> GSEFVKEHDWKKCDQSGFCRRNRAYADHALSAISWESPYKIAPETGSFKDGQYQAIILKTINDHGETVRLPLTVSFLESGTARVTIDEEKRQKGEIELRHDSKARKERYNEAEQWVIVGGMTLDKGAKVDYEDKTQMTVKYGPSSKFEATIKFAPFSIDFKRDGASHIKFNDQGLLNIEHWRPKIDPPPEPEKKEGEQQPDKKEEAPREDDSTWWEESFGGNTDSKPRGPESVGLDISFVGYEHVFGIPSHASPLSLKQTRGGEGNYNEPYRMYNADVFEYILDSPMTLYGSIPFMQAHRKDSSVGIFWLNAAETWVDITKGKDSKNPLALGVKSKITTRTHWFSESGLLDVFVFLGPTPKDIISKYAELTGTTAMPQEFSLGYHQCRWNYVSDEDVKDVDRKMDKFNMPYDVIWLDIEYTDEKKYFTWDKHSFKDPIGMGKQLEAHGRKLVTIIDPHIKNTNNYPVVDELKSKDLAVKTKDGSIFEGWCWPGSSHWIDAFNPAAREWWKGLFKYDKFKGTMENTFIWNAMNEPSVFNGPEVTMPKDNLHHGNWEHRDVHNLNGMTFQNATYHALLSRKPGEHRRPFVLTRAFFAGSQRLGAMWTGDNTADWGYLKASIPMVLSQGIAGFPFAGADVGGFFGNPDKDLLTRWYQTGIFYPFFRAHAHIDARRREPYLTGEPYNTIIAAALRLRYSLLPSWYTAFRHAHLDGTPIIKPMFYTHPSEEAGLPIDDQFFIGNTGLLAKPVTDKDRTSVDIWIPDSEVYYDYFTYDIISAAKSKTATLDAPLEKIPLLMRGGHVFARRDIPRRSSALMKWDPYTLVVVLGNDRKAEGDLYVDDGDSFDYEKGQYIHRRFIFDANTLTSADYEGRDDASIKEGEWLKKMRTVNVEKIIVVGAPAAWKGKKTVTVESEGKTWAAAIEYNPAEKSRAAFAVVKKVGVRVGADFKIVFG

Glucosidase I removes the outermost α1,2-linked glucose from the D1 branch, and then glucosidase II (GII) trims second and third α1,3-linked glucose residues by catalyzing hydrolyses at the Glc-α1,3-Glc and Glc-α1,3-Man glycosidic linkages. Here we performed an X-ray crystallographic study of GIIα to elucidate its substrate recognition mechanism. The overall structure of GIIα is composed of four major domains and three subdomains: N-terminal domain (residues 31–384), subdomain B1 (residues 207–256), β8α8 barrel domain (residues 385–737), subdomain B2 (residues 484–526), subdomain B3 (residues 559–581), proximal C-terminal domain (residues 738–823), and distal C-terminal domain (residues 824–977). Taken together, our structural data revealed that GIIα can recognize two kinds of glucosylated substrates, Glc-α1,3-Glc and Glc-α1,3-Man, via a bilocular substrate-binding pocket with a tolerant +1 subsite.

To elucidate the two-step enzymatic reaction mechanisms of GII, we performed the structural determination of substrate-bound complexes of GIIα using its inactive mutant in which the catalytic residue Asp556 was substituted with alanine. We used Glc-α1,3-Glc (α3-Glc2) and Glc-α1,3-Man-α1,2-Man (Glc1Man2) corresponding to Glc(G2)-Glc(G3) and Glc(G3)-Man(D1)-Man(C) in Glc3Man9GlcNAc2, respectively. The final model of the α3-Glc2-bound GIIα refined to 2.40 Å resolution has an Rwork of 14.8% and Rfree of 19.9%, whereas that of the Glc1Man2-bound form refined to 2.30 Å resolution has an Rwork of 14.4% and Rfree of 18.9%. The α3-Glc2 ligand containing the scissile bond of the first reaction of GII was accommodated in a gourd-shaped bilocular pocket. Two glucose residues were clearly visible in the electron density map and were traced as Glc-α1,3-Glc. The disaccharide ligand binds to the pocket with the nonreducing terminal Glc(G2) residue interacting with the deeply buried −1 subsite and the reducing Glc(G3) occupying the surface-proximal +1 subsite, explaining its exo-α1,3-glucosidase activity. In the −1 subsite, all the hydroxyl groups of the Glc(G2) residue interacted with Asp443, Arg617, Asp633, and His691. Additionally, Asp482, Trp517, Trp630, and Asp662 formed hydrogen bonds via water molecules, and Trp415 formed a hydrophobic interaction. In the +1 subsite, the 4-OH and 6-OH groups of the glucose residue form hydrogen bonds with Asp303 (N-loop) and Arg617. In the Glc(G2)-Glc(G3)-bound complex, the equatorial 2-OH group of Glc(G3) is not involved in interaction, whereas the axial 2-OH group of Man(D1) forms a hydrogen bond with Asp633 in the Glc(G3)-Man(D1)-bound complex, suggesting its contribution to enhanced affinity.>MDKKSRVLIVGGTGYIGKRIVNASISLGHPTYVLFRPEVVSNIDKVQMLLYFKQLGAKLIEASLDDHQRLVDALKQV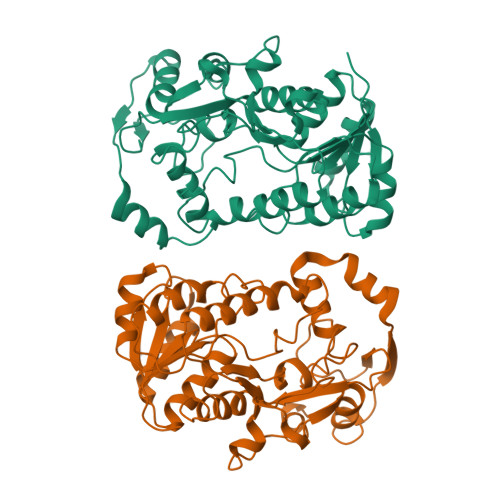DVVISALAGGVLSHHILEQLKLVEAIKEAGNIKRFLPSEFGMDPDIMEHALQPGSITFIDKRKVRRAIEAASIPYTYVSSNMFAGYFAGSLAQLDGHMMPPRDKVLIYGDGNVKGIWVDEDDVGTYTIKSIDDPQTLNKTMYIRPPMNILSQKEVIQIWERLSEQNLDKIYISSQDFLADMKDKSYEEKIVRCHLYQIFFRGDLYNFEIGPNAIEATKLYPEVKYVTMDSYLERYV[4x]>[4x]MVVMEEIIKKAFIESINNIRRGDKEEELKKIQEKIVNAKKIV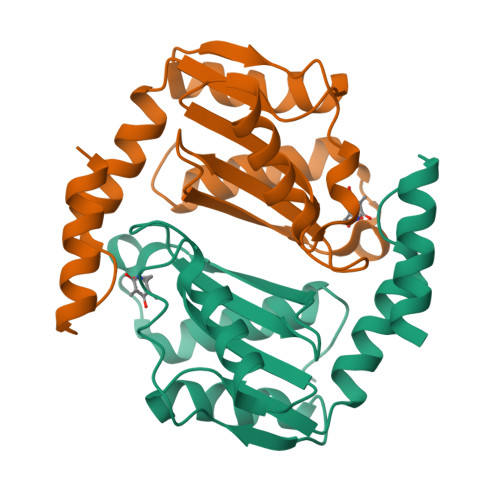VATNNQKKFKVIRDIMLRVCNAEIKMLDIDTRFADLTRMPALTKGLIALDIEKADLYIARGRLGAPGSGSMLVILDEKGRVLTASLSPSSVIHKEDIEERIKKELIEALSRIGISILEHHHHHH>[2x]HGSVVDPASRNYGCWLRWGDDFQNPAMEQEDPMCWQAWQADPNAMWNWNGLYRNGSGGDFPAAVPDGQLCSGGRTES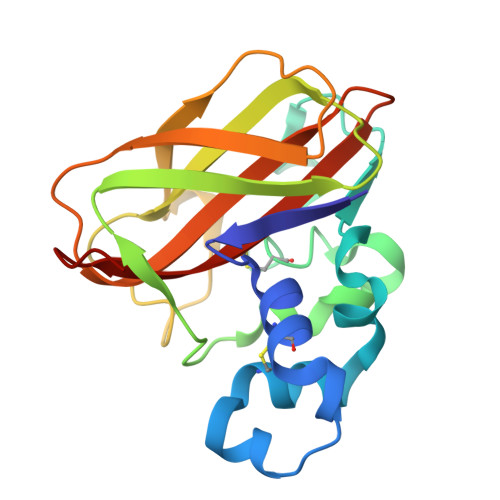GRYDSLDSVGAWKTTDITDDFTVKLYDQASHGADYFQVYVTRQGFDPAAEALTWSDLQLVAETGRYAPSQNYEIPVTTSGLSGRHVVYTIWQASHMDQTYFLCSDVNFTHHHHHH> DISSTEIAVYWGQREDGLLRDTCKTNNYKIVFISFLDKFGCEIRKPELELEGVCGPSVGNPCSFLESQIKECQRMGVKVFLALGGPKGTYSACSADYAKDLAEYLHTYFLSERREGPLGKVALDGIHFDIQKPVDELNWDNLLEELYQIKDVYQSTFLLSAAPGCLSPDEYLDNAIQTRHFDYIFVRFYNDRSCQYSTGNIQRIRNAWLSWTKSVYPRDKNLFLELPASQATAPGGGYIPPSALIGQVLPYLPDLQTRYAGIALWNRQADKETGYSTNIIRYLNATAMPFTSNLLKYPS

The European XFEL (EuXFEL) in Germany is the first MHz XFEL. Our results demonstrate that MHz XFELs can be used to collect high-quality serial femtosecond crystallography data, and that under the conditions used in the current experiment, shock waves caused by the interaction between the sample jet and the XFEL pulses do not compromise the data to a measurable extent. We demonstrate here that it is possible to separate the data of the three types of protein crystals in such a microcrystalline mixture of jack bean proteins (urease, concanavalin A and B), and to determine the structures of the two concanavalins, using data collected at the first MHz XFEL. Therefore, now that the first MHz XFEL has become available, we investigated this issue at current EuXFEL operating parameters, using microcrystals of the model protein lysozyme.

As well as addressing the challenges associated with MHz data repetition rates using a model system (lysozyme protein crystals), we investigated a microcrystalline preparation of jack bean proteins precipitated with acetone, a preparation described by James Sumner, who used this technique for the first crystallization of an enzyme (urease) in 192618, resulting in a Nobel Prize in 194619. To this end, we collected SFX data of a microcrystalline mixture of jack bean proteins, crystallized using acetone as published previously. The microcrystalline slurry contained at least three different crystal forms. Due to their small size (on the order of 5–10 μm) the crystals could not be further characterized before the beam time and it thus remained unclear which proteins had in fact crystallized. In contrast to the concanavalin A and B microcrystals, which diffracted strongly, urease microcrystals diffracted only to low resolution and with low signal-to-noise ratio, and no structure was refined. Indeed, the electron density maps are of excellent quality and the overall structures are virtually identical to those determined using macroscopic crystals, with core RMSDs on Cα atoms against reference structures of 0.31 Å for concanavalin A (vs. PDB entry 1JBC30) and 0.24 Å for concanavalin B (vs. PDB entry 1CNV31). Given the lysozyme results, it appears unlikely that our jack bean protein data are compromised by radiation damage or by shock wave effects in the current experiment. As shown by the electron density maps of the concanavalin A and B structures determined in this study, the data are of high quality and this is likely to improve as experience with ultrafast detectors such as the AGIPD increases. Moreover, in just one shift (12 h) of data collection, ~77,000 indexed images were collected of concanavalin A and ~24,000 of concanavalin B, despite this being one of the very first experiments at a new facility.>MSWQAYVDDHLMCEIEGNHLSAAAIIGQDGSVWAQSANFPQFKSEEITGIMSDFHEPGTLAPTGLYIGGTKYMVIQGEPGAVIRGKKGPGGVTVKKTNQALI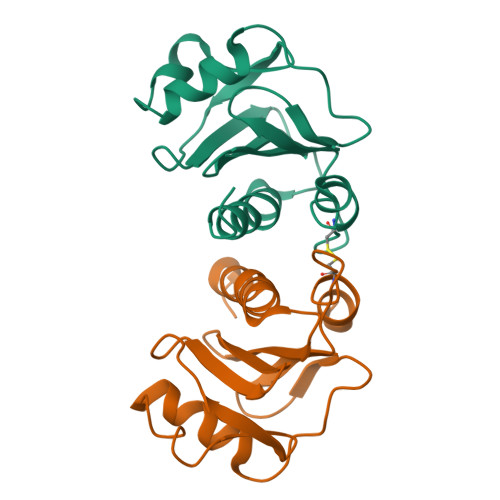IGIYDEPMTPGQCNMIVERLGDYLIDQGY[2x]>GAMADREKLLTESGVYGTFATFQMDHDWWDLPGESRVISVAEVKGLVEQWSGKILVESYLLRGLSDHADLMFRVHARTLSDTQQFLSAFMGTRLGRHLTSGGLLHGVSKKPTYVAGFPESMKTELQVNGESGSRPYAIVIPIKKDAEWWALDQEARTALMQEHTQAALPYLKTVKRKLYHSTGLDDVDFITYFETERLEDFHNLVRALQQVKEFRHNRRFGHPTLLGT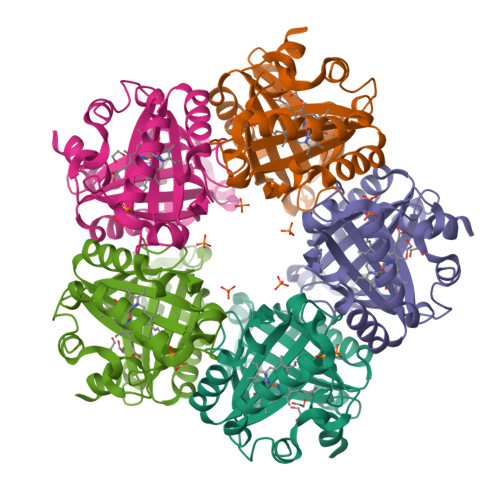MSPLDEILEKFAQ[5x]> GMTGAVETESMKTVRIREKIKKFLGDRPRNTAEILEHINS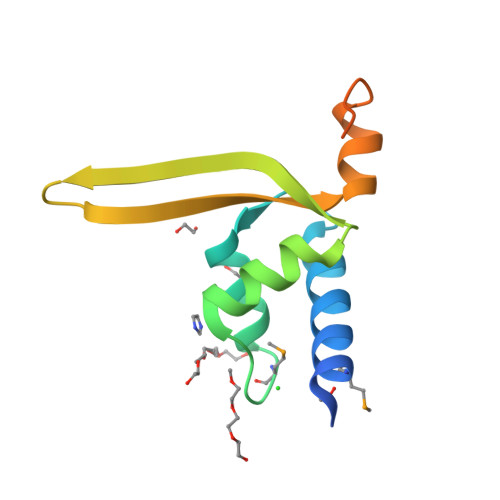TMRHGTTSQQLGNVLSKDKDIVKVGYIKRSGILSGGYDICEWATRNWVAEHCPEWTEGQPIILNEEGDFTLGPLPE>[2x]V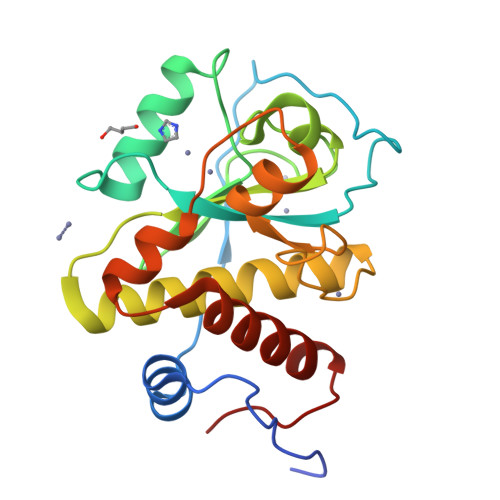SSQKTSSLPKYTPKVNSSINNYIRKKNMKAPRIEEDYTSYFPKYGYRNGVGRPEGIVVHDTANDNSTIDGEIAFMKRNYTNAFVHAFVDGNRIIETAPTDYLSWGAGPYGNQRFINVEIVHTHDYDSFARSMNNYADYAATQLQYYNLKPDSAENDGRGTVWTHAAISNFLGGTDHADPHQYLRSHNYSYAELYDLIYEKYLIKTKQVAPWG> MKPPRPVRTCSKVLVLLSLLAIHQTTTAEKNGIDIYSLTVDSRVSSRFAHTVVTSRVVNRANTVQEATFQMELPKKAFITNFSMIIDGMTYPGIIKEKAEAQAQYSAAVAKGKSAGLVKATGRNMEQFQVSVSVAPNAKITFELVYEELLKRRLGVYELLLKVRPQQLVKHLQMDIHIFEPQGISFLETESTFMTNQLVDALTTWQNKTKAHIRFKPTLSQQQKSPEQQETVLDGNLIIRYDVDRAISGGSIQIENGYFVHYFAPEGLTTMPKNVVFVIDKSGSMSGRKIQQTREALIKI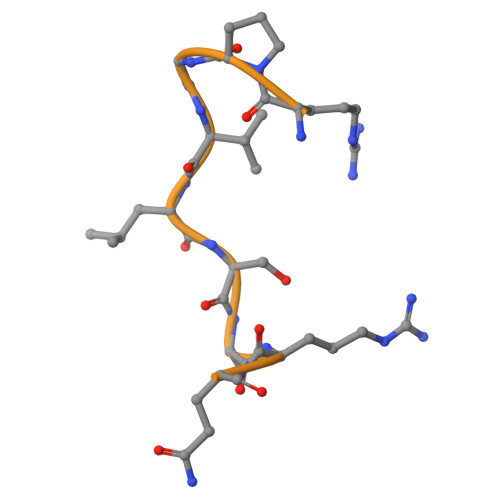LDDLSPRDQFNLIVFSTEATQWRPSLVPASAENVNKARSFAAGIQALGGTNINDAMLMAVQLLDSSNQEERLPEGSVSLIILLTDGDPTVGETNPRSIQNNVREAVSGRYSLFCLGFGFDVSYAFLEKLALDNGGLARRIHEDSDSALQLQDFYQEVANPLLTAVTFEYPSNAVEEVTQNNFRLLFKGSEMVVAGKLQDRGPDVLTATVSGKLPTQNITFQTESSVAEQEAEFQSPKYIFHNFMERLWAYLTIQQLLEQTVSASDADQQALRNQALNLSLAYSFVTPLTSMVVTKPDDQEQSQVAEKPMEGESRNRNVHSGSTFFKYYLQGAKIPKPEASFSPRRGWNRQAGAAGSRMNFRPGVLSSRQLGLPGPPDVPDHAAYHPFRRLAILPASAPPATSNPDPAVSRVMNMKIEETTMTTQTPAPIQAPSAILPLPGQSVERLCVDPRHRQGPVNLLSDPEQGVEVTGQYEREKAGFSWIEVTFKNPLVWVHASPEHVVVTRNRRSSAYKWKETLFSVMPGLKMTMDKTGLLLLSDPDKVTIGLLFWDGRGEGLRLLLRDTDRFSSHVGGTLGQFYQEVLWGSPAASDDGRRTLRVQGNDHSATRERRLDYQEGPPGVEISCWSVEL> MGSSHHHHHHSQSPMFDIKRKTIEWGGKTLVLETGRIARQADGAVLATMGETVVLATAVFAKSQKPGQDFFPLTVNYQEKTFAAGKIPGGFFKREGRPSEKETLVSRLIDRPIRPLFVKGFKNEVQVVVTVLQHDLENDPDILGMVAASAALCLSGAPFMGPIGAARVGWVDGAYVLNPTLDEMKESKMDLVVAGTADAVMMVESEIQELSEEIVLGGVNFAHQQMQAVIDAIIDLAEHAAKEPFAFEPEDTDAIKAKMKDLVGADIAAAYKIQKKQDRYEAVGAAKKKAIAALGLSDENPTGYDPLKLGAIFKELEADVVRRGILDTGLRIDGRDVKTVRPILGEVGILPRTHGSALFTRGETQAIVVATLGTGDDEQFIDALEGTYKESFLLHYNFPPYSVGETGRMGSPGRREIGHGKLAWRALRPMLPTKEDFPYTIRLVSEITESNGSSSMATVCGSSLAMMDAGVPLVRPVSGIA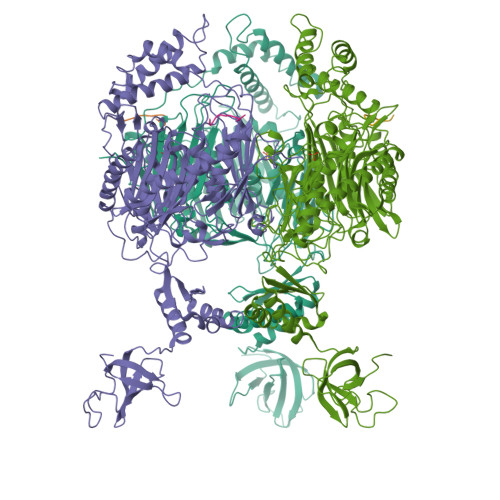MGLILEQDGFAVLSDILGDEDHLGDMDFKVAGTSEGLTSLQMDIKIAGITPAIMEQALAQAKEGRAHILGEMNKAMDAPRADVGDFAPKIETINIPTDKIREVIGSGGKVIREIVATTGAKVDINDDGVVKVSASDGAKIKAAIDWIKSITDEAEIGKIYDGKVVKVVDFGAFVNFFGAKDGLVHVSQISNERVAKPSDVLKEGQMVKVKLLGFDDRGKTKLSMKVVDQETGEDLSKKEAAAEEA;> TAPPEKPRRGWWRR> MFLTAEDCFELGKVAYTEADYYHTELWMEQALRQLDEGE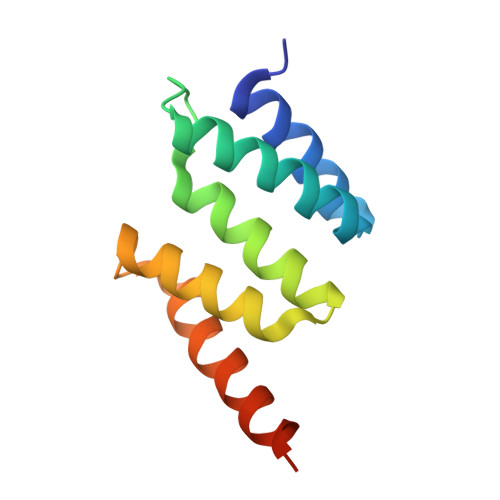ISTIDKVSVLDYLSYAVYQQGDLDKALLLTKKLLELDPEHQRANGNLKYFEYIMAKEKDVNKSAS>MHNHNHNHNHNHNGGENLYFQGASLTEIEHLVQSVCKSYRETCQLRLEDLLRQRSNIFSREEVTGYQRKSMWEMWERCAHHLTEAIQYVVEFAKRLSGFMELCQNDQIVLLKAGAMEVVLVRMCRAYNADNRTVFFEGKYGGMELFRALGCSELISSIFDFSHSLSALHFSEDEIALYTALVLINAHRPGLQEKRKVEQLQYNLELAFHHHLCKTHRQSILAKLPPKGKLRSL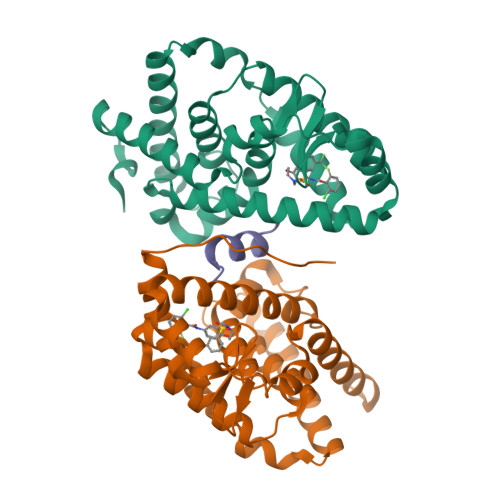CSQHVERLQIFQHLHPIVVQAAFPPLYKELFS[2x];> VERLQIFQHLHPI> MDGPGASAVVVRVGIPDLQQTKCLRLDPTAPVWAAKQRVLCALNHSLQDALNYGLFQPPSRGRAGKFLDEERLLQDYPPNLDTPLPYLEFRYKRRVYAQNLIDDKQFAKLHTKANLKKFMDYVQLHSTDKVARLLDKGLDPNFHDPDSGECPLSLAAQLDNATDLLKVLRNGGAHLDFRTRDGLTAVHCATRQRNAGALTTLLDLGASPDYKDSRGLTPLYHSALGGGDALCCELLLHDHAQLGTTDENGWQEIHQACRFGHVQHLEHLLFYGANMGAQNASGNTALHICALYNQESCARVLLFRGAN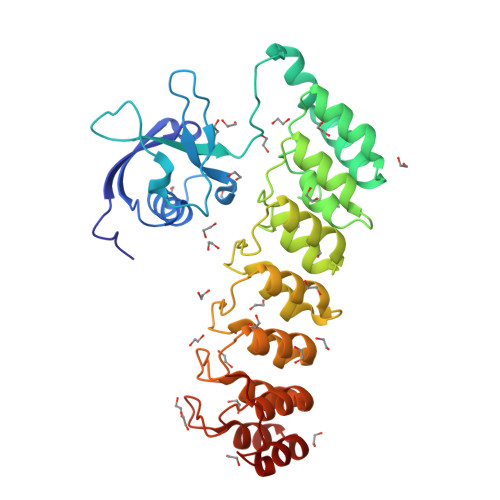KDVRNYNSQTAFQVAIIAGNFELAEVIKTHKDSDVVPFRE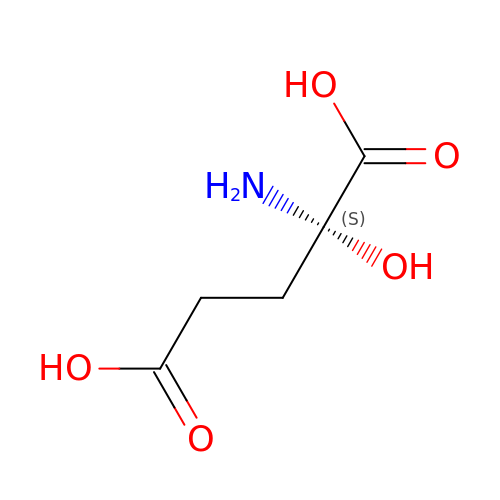(2S)-2-azanyl-2-oxidanyl-pentanedioic acid | C5 H9 N O5 | GXSDWXSYZHGBBO-YFKPBYRVSA-N(3AS,5S,6S,7R,7AR)-5-FLUORO-5-(HYDROXYMETHYL)-2-METHYL-5,6,7,7A-TETRAHYDRO-3AH-PYRANO[3,2-D][1,3]OXAZOLE-6,7-DIOL 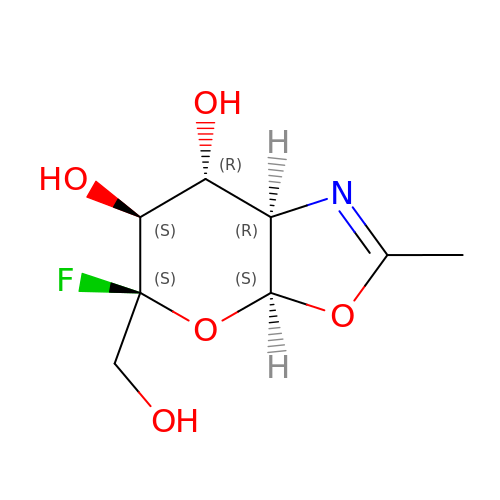| C8 H12 F N O5 | GCSIDVFZDNBNLE-QQGCVABSSA-N~{N}-[2-[[(2~{S})-3-[[(2~{S})-3-[[1-[2-[2-[2-[4-[4-[5-(acetamidomethyl)-2-oxidanylidene-1,3-oxazolidin-3-yl]-2-fluoranyl-phenyl]piperazin-1-yl]-2-oxidanylidene-ethoxy]ethoxy]ethyl]-1,2,3-triazol-4-yl]methylamino]-2-[[2,3-bis(oxidanyl)phenyl]carbonylamino]-3-oxidanylidene-propyl]amino]-2-[[2,3-bis(oxidanyl)phenyl]carbonylamino]-3-oxidanylidene-propyl]amino]-2-oxidanylidene-ethyl]-2,3-bis(oxidanyl)benzamide 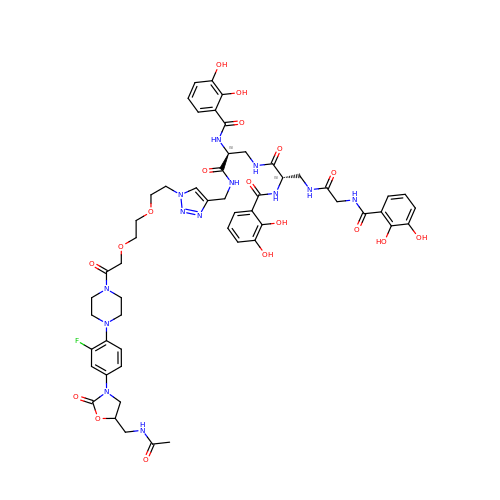| C54 H62 F N13 O18 | OQJXSZUYGZCTKY-ACLHFTIQSA-N Different AAF variants are expressed by different EAEC strains, where they are required for the bacterium's adherence to small and large intestinal mucosa. As with Afa/Dr polyadhesins, AAF consist of two secreted protein subunits, a major subunit (A) and a putative minor subunit (B). In the fiber, subunits are linked together by donor strand complementation (DSC) with an N-terminal Gd donor strand segment of one subunit inserted into the hydrophobic cleft of a neighboring subunit. In this study, we report X-ray crystallographic and NMR studies of monomeric, donor-strand-complemented major and minor subunits of AAF/I from the German outbreak strain and AAF/II from EAEC strain 042 and provide an atomic resolution model for the structure of the entire fimbriae.

The minor subunits AggBdsA and AafBdsA have more similar structures than the major pilins: 117 matching Cα atoms are superimposed with r.m.s.d. of 1.2 Å. The donor sequences derived from the corresponding major subunits form classical donor strands (Gd), each inserting five donor residues into the subunit core structure. As predicted, the minor subunits have no N-terminal extension that could act as a donor strand: the first residue in the mature protein is structured and immediately followed by the first strand A. Hence, this structural evidence suggests that the minor subunits assemble by accepting donor sequences of the corresponding major subunits. As such sequences are only available in tip subunits of major subunit polymers, the AAF minor subunits are likely to be tip localized. Furthermore, the significant sequence identity with the AfaD tip invasin (>60%),which has been visualized as a tip subunit, together with the ability of AggB to functionally complement AfaD mutants are also suggestive of a similar localization for AAF minor sununits. In minor subunits, strand A is not split between the β sheets, but locates entirely in the sheet 1. Instead, strand C2 that in a classical Ig fold is hydrogen bonded to strand F, in minor subunits is hydrogen bonded to strand D and hence belongs to sheet 2. A conserved disulfide bond also stabilizes the minor subunits. However, this bond connects the BC1 loop with the end of strand F and not the beginning of the fold as in major subunits. Interestingly, AggBdsA also bound to fibronectin but with significantly lower affinity (∼100 µM).

>[8x]AEITLISHKTLGSQLRDGMKLATGRIACREPHDGFHIWINASQNGKVGHYIVQNNRETKHELKVKIGGGGWSSSLIEGQRGVYRQGEEKQAIFDIMSDGNQYSAPGEYIFSVSGECLISRGDNKQALERPPIKATETIRLTV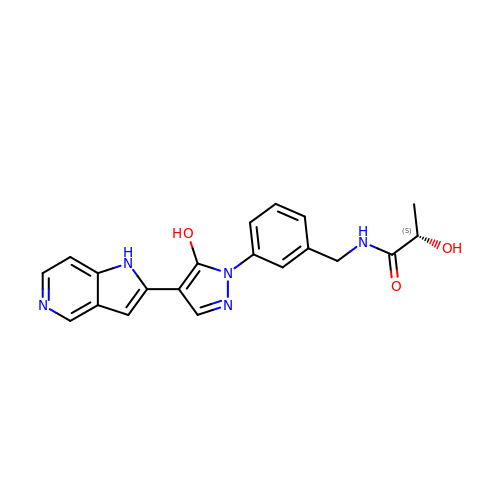(2S)-2-hydroxy-N-[[3-[5-hydroxy-4-(1H-pyrrolo[3,2-c]pyridin-2-yl)pyrazol-1-yl]phenyl]methyl]propanamide | C20 H19 N5 O3 | DDFTUZONFSKIPC-LBPRGKRZSA-N> GHMNIQSTIKAVAETISTGPIPGSRKVYQAGELFPELRVPFREVAVHPSANEPPVTIYDPSGPYSDPAIQIDIEKGLPRTREALVVARGDVEEVADPRQVKPEDNGFAQGKHLAPEFPDTGRKIYRAKPGKLVTQLEYARAGIITAEMEYVAIRENLRREQDRPCVRDGEDFGASIPDFVTPEFVRQEIARGRAIIPANINHGELEPMAIGRNFLVKINANIGNSAVLSTVADEVDKLVWATRWGADTVMDLSTGRNIHNIRDWIIRNSSVPIGTVPIYQALEKVNGVAEDLNWEVFRDTLIEQCEQGVDYFTIHAGVRLPFIPMTAKRVTGIVSRGGSIMAKWCLAHHKENFLYERFDEICEIMRAYDVSFSLGDGLRPGSTADANDEAQFSELRTLGELTKVAWKHGVQVMIEGPGHVAMHKIKANMDEQLKHCHEAPFYTLGPLTTDIAPGYDHITSAIGAAMIGWFGTAML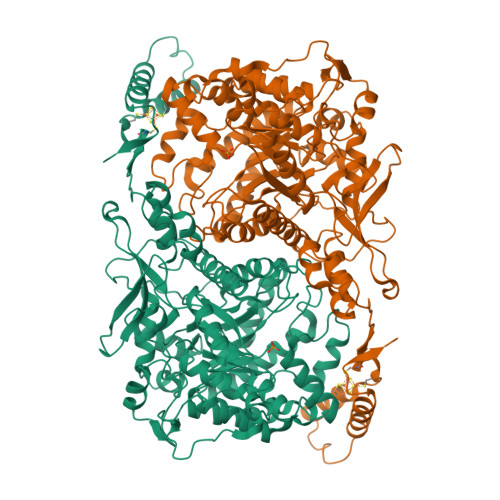CYVTPKEHLGLPDRDDVKTGVITYKLAAHAADLAKGHPGAAMWDDAISRARFEFRWEDQFNLGLDPETARKFHDETLPKEAHKTAHFCSMCGPKFCSMKISQEVRDFAAGKAPNSAELGMAEMSEKFREQGSEIYLKTE> AGITGTWYNQLGSTFIVTAGADGALTGTYESAVGNAESRYVLTGRYDSAPATDGSGTALGWTVAWKNNYRNAHSATTWSGQYVGGAEARINTQWLLTSGTTEANAWKSTLVGH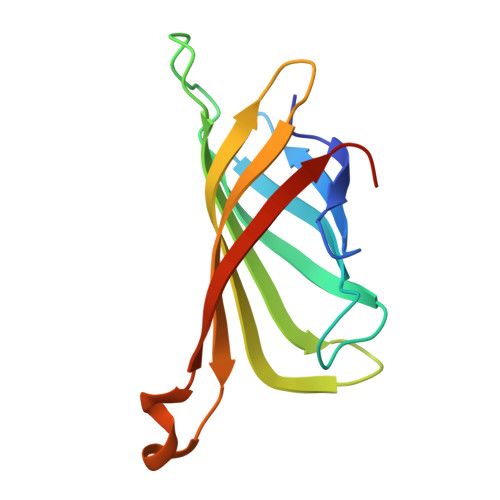DTFTKVKPSAA>[2x]GAMTGSSKFEEFMTRHQVHEKEEFKALKTLSIFYQAGTSKAGNPIF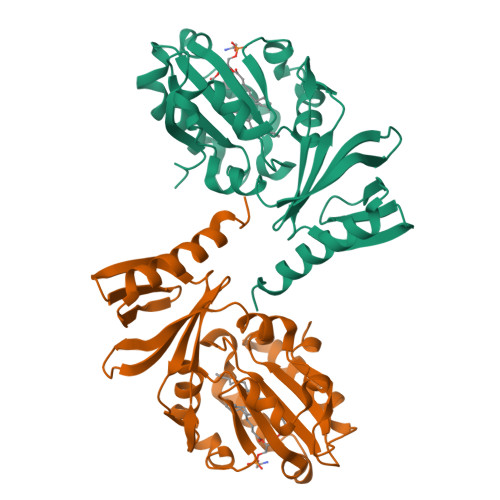YYVARRFKTGQINGDLLIYHVLLTLKPYYAKPYEIVVDLTHTGPSNRFKTDFLSKWFVVFPGFAYDNVSAVYIYNCNSWVREYTKYHERLLTGLKGSKRLVFIDCPGKLAEHIEHEQQKLPAATLALEEDLKVFHNALKLAHKDTKVSIKVGSTAVQVTSAERTKVLGQSVFLNDIYYASEIEEICLVDENQFTLTIANQGTPLTFMHQECEAIVQSIIHIRTRWELSQPD>MAKKTSSKGKLPPSPKPRLPFIGHLHLLDNPLLHHTLIKLGKRYGPLYTLYFGSMPTVVASTPDLFKLFLQTHEATSFNTRFQTSAISRLTYDNSVAMVPFAPYWKFIRKLIMNDLLNATTVNKLRPLRSREILKVLKVMANSAETQQPLDVTEELLKWTNSTISTMMLGEAEEVRDIARDVLKIFGEYSVTNFIWPLNKFKFGNYDKRTEEIFNKYDPIIEKVIKKRQEIVNKRKNGEIVEGEQNVVFLDTLLEFAQDETMEIKITKEQIKGLVVDFFSAGTDSTAVSTEWTLSELINNPRVLKKAREEIDSVVGKDRLVDESDVQNLPYIKAIVKEAFRLHPPLPVVKRKCTQECEIDGYVVPEGALILFNVWAVGRDPKYWVKPLEFRPERFIENVGEGEAASIDLRGQHFTLLPFGSGRRMCPGVNLATAGMATMIASIIQCFDLQVPGQHGEIL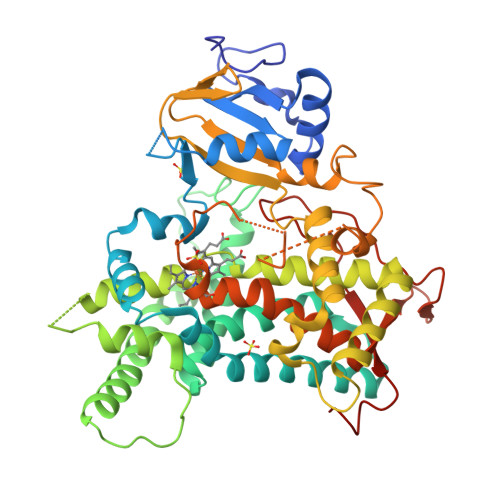NGDYAKVSMEERPGLTVPRAHNLMCVPLARAGVADKLLSSHHHH[2x]> AALFQEQAERSEKLRTESYQDNLTGLANRRYFEMQLNARVSNPEQASSGYLLLLRVKDLAGLNQRLGGQRTDELLKAVGEQLSRECAKYPETQNLVTRIRGGEFAVLAPGMTREEALQLAQSLDSALSSLYATGATDVAAVASIGLAPFAHGDSPQAVLSLGDQALAQAEGQGEQNWACLDQSLVADVGDDHHAWHRLLDQALNQRRFELFFQPVVAAQDTQLVLHYKVLSRLLDEQGQTIPAGRFLPWLERFGWTARLDRLMLERVLEQMAGHEESLALNLSSATLADPQALNKVFEILRAHSNLGARLTLEIGEEQLPEQAVLEQLTRRLRELGFSLSLQRFGGRFSMIGNLARLGLAYLKIDGSYIRAIDQESDKRLFIEAIQRAAHSIDL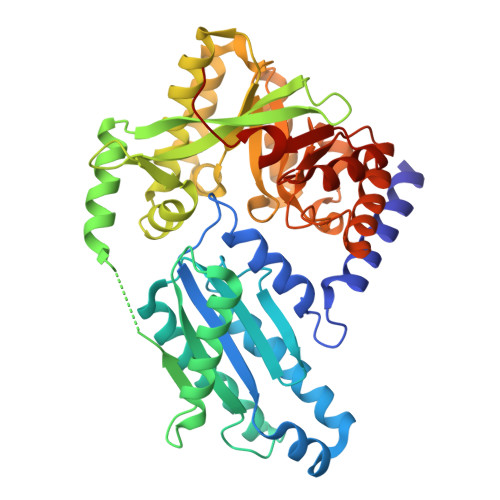PLIAERVETEGELSVIREMGLYGVQGQLFGEPKPWG6-(4-chlorophenyl)-1-methyl-5-[(3S)-1-methyl-2-oxo-2,3-dihydro-1H-indol-3-yl]-1H-pyrrolo[2,3-d]pyrimidine-2,4(3H,7H)-dione 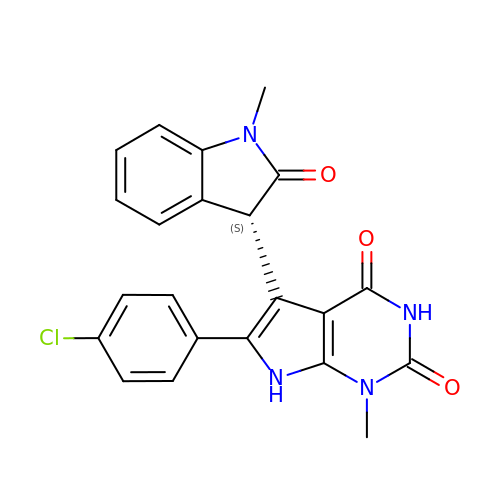| C22 H17 Cl N4 O3 | AHQASKURDHESBQ-HNNXBMFYSA-N> GGACAUAUAAUCGCGUGGAUAUGGCACGCAAGUUUCUACCGGGCACC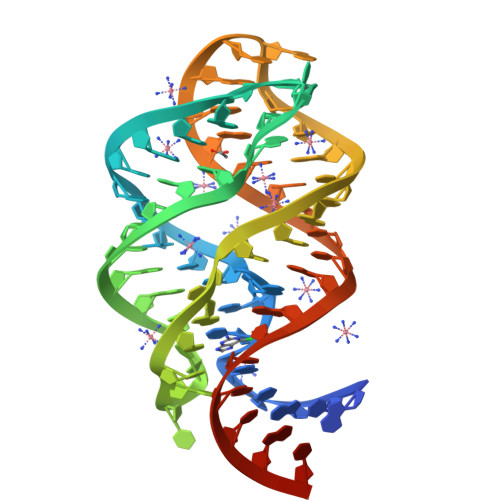GUAAAUGUCCGAUUAUGUCCA>GSHMSHAPTRSARDIHQLEARIDSLAARNSKLMETLKEAR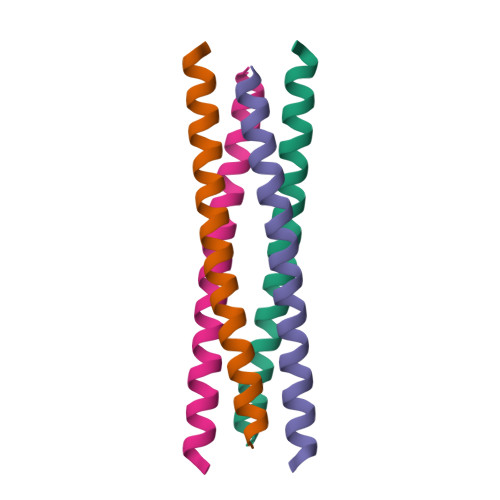QQLLALREEVDRLGQ[6x]> MERTNTTTFKFFSLGGSNEVGRSCHILQYKGKTVMLDAGIHPAYQGLASLPFYDEFDLSKVDILLISHFHLDHAASLPYVMQRTNFQGRVFMTHPTKAIYRWLLRDFVRVTSIGSSSSSMGTKDEGLFSDEDLVDSFDKIETVDYHSTVDVNGIKFTAFHAGHVLGAAMFQIEIAGLRVLFTGDYSREVDRHLNSAEVPPLSSNVLIVESTFGTATHEPRLNRERKLTQLIHSTVMRGGRVLLPVFALGRAQEIMLILDEYWSQHADELGGGQVPIFYASNLAKKCMSVFQTYVNMMNDDIRKKFRDSQTNPFIFKNISYLRNLEDFQDFGPSVMLASPGMLQSGLSRDLLERWCPEDKNLVLITGYSIEGTMAKFIMLEPDTIPSINNPEITIPRRCQVEEISFAAHVDFQENLEFIEKISAPNIILVHGEANPMGRLKSALLSNFASLKGTD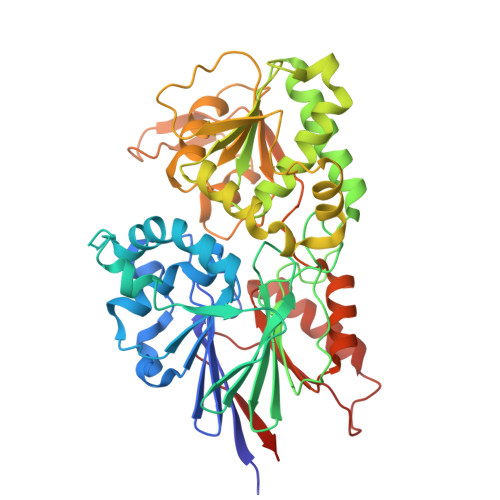NEVHVFNPRNCVEVDLEFQG>[3x]MASGSMHLRPIATPYPVKEWLQPKRYKAHLMGTTYVYDFPELFRQASSSQWKNFSADVKLTDDFFISNELIEDENGELTEVEREPGANAIGMVAFKITVKTPEYPRGRQFVVVANDITFKIGSFGPQEDEFFNKVTEYARKRGIPRIYLAANSGARIGMAEEIVPLFQVAWNDAANPDKGFQYLYLTSEGMETLKKFDKENSVLTERTVINGEERFVIKTIIGSEDGLGVECLRGSGLIAGATSRAYHDIFTITLVTCRSVGIGAYLVRLGQRAIQVEGQPIILTGAPAINKMLGREVYTSNLQLGGTQIMYNNGVSHLTAVDDLAGVEKIVEWMSYVPAKRNMPVPILETKDTWDRPVDFTPTNDETYDVRWMIEGRETESGFEYGLFDK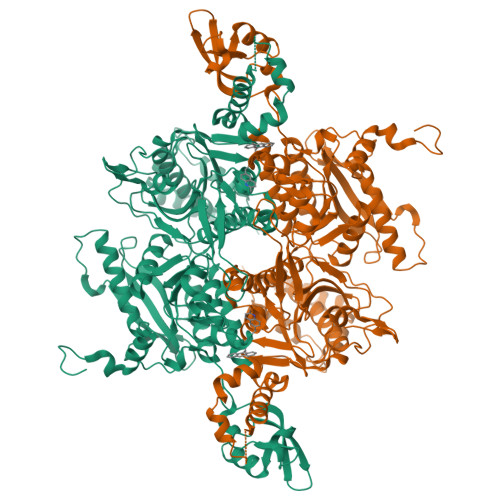GSFFETLSGWAKGVVVGRARLGGIPLGVIGVETRTVENLIPADPANPNSAETLIQEPGQVWHPNSAFKTAQAINDFNNGEQLPMMILANWRGFSGGQRDMFNEVLKYGSFIVDALVDYKQPIIIYIPPTGELRGGSWVVVDPTINADQMEMYADVNARAGVLEPQGMVGIKFRREKLLDTMNRLDDKYRELRSQLSNKSLAPEVHQQISKQLADRERELLPIYGQISLQFADLHDRSSRMVAKGVISKELEWTEARRFFFWRLRRRLNEEYLIKRLSHQVGEASRLEKIARIRSWYPASVDHEDDRQVATWIEENYKTLDDKLKGLKLESFAQDLAKKIRSDHDNAIDGLSEVIKMLSTDDKEKLLKTLKLEHHHHHH> MSEKHPGPLVVEGKLTDAERMKHESNYLRGTIAEDLNDGLTGGFKGDNFLLIRFHGMYQQDDRDIRAERAEQKLEPRHAMLLRCRLPGGVITTKQWQAIDKFAGENTIYGSIRLTNRQTFQFHGILKKNVKPVHQMLHSVGLDALATANDMNRNVLCTSNPYESQLHAEAYEWAKKISEHLLPRTRAYAEIWLDQEKVATTDEEPILGQTYLPRKFKTTVVIPPQNDIDLHANDMNFVAIAENGKLVGFNLLVGGGLSIEHGNKKTYARTASEFGYLPLEHTLAVAEAVVTTQRDWGNRTDRKNAKTKYTLERVGVETFKAEVERRAGIKFEPIRPYEFTGRGDRIGWVKGIDDNWHLTLFIENGRILDYPARPLKTGLLEIAKIHKG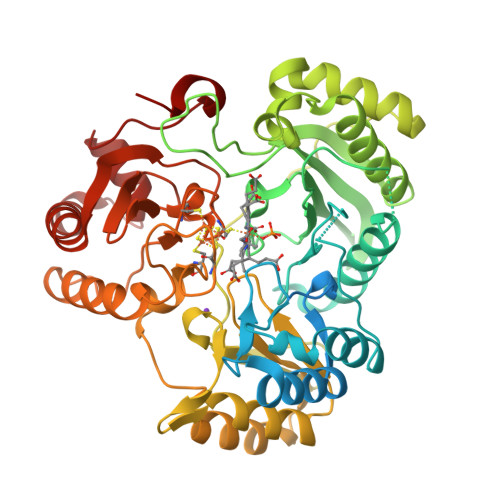DFRITANQNLIIAGVPESEKAKIEKIAKESGLMNAVTPQRENSMACVSFPTCPLAMAEAERFLPSFIDNIDNLMAKHGVSDEHIVMRVAGCPNGCGRAMLAEVGLVGKAPGRYNLHLGGNRIGTRIPRMYKENITEPEILASLDELIGRWAKEREAGEGFGDFTVRAGIIRPVLDPARDLWD> DELYRQSLEIISRYLREQATGAKDTKPMGRSGATSRKALETLRRVG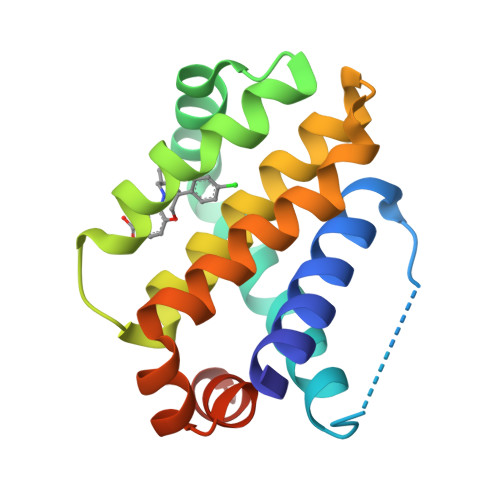DGVQRNHETAFQGMLRKLDIKNEDDVKSLSRVMIHVFSDGVTNWGRIVTLISFGAFVAKHLKTINQESCIEPLAESITDVLVRTKRDWLVKQRGWDGFVEFFHVEDLEGG SWELL1 or LRRC8a (leucine-rich repeat-containing protein 8a) encodes a transmembrane protein first described in 2003 as the site of a balanced translocation in an immunodeficient child with agammaglobulinemia and absent B-cells. So, for about a decade, SWELL1 was considered a membrane protein that regulates PI3K-AKT mediated lymphocyte function, and it was not until 2014 that SWELL1/LRRC8a was discovered to also form an essential component of the volume-regulated anion channel (VRAC), forming hetero-hexamers with LRRC8b-e22,23. We previously showed SWELL1 to mediate insulin-PI3K-AKT signaling in adipocytes, skeletal muscle, and endothelium via non-conductive signaling mechanisms. Also, we and others showed SWELL1-LRRC8 channel activity (conductive signaling) in the pancreatic β-cell is required for normal insulin secretion.

Additional binding interactions for SN-403, SN-406 and SN-407 are also predicted along the channel, due to the longer carbon chains affording additional hydrophobic interactions with side-chain carbons of the R103 residues (purple dashes). As anticipated, SN-403, SN-406, and SN-407 had increased ICl,SWELL inhibitory activity compared to SN-401, with SN-406 and SN-407 having IC50 of 3.1 and 1.6 μM, respectively, and SN-401 IC50 = 3.9 μM. In initial maps using sixfold symmetry, SN-407 density was less apparent than for DCPIB/SN-40131, potentially due to a reduction in SN-407 occupancy that is a consequence of lower compound solubility or the presence of multiple drug poses in different particles. In Pose-2, SN-407 is tilted off the SWELL1 central axis, positioning its cyclopentyl group closer to the hydrophobic cleft between SWELL1 subunits. These data confirm lengthening the carboxylate chain in SN-407 preserves electrostatic interactions with R103 and enables additional contacts between the carboxylate chain and upper hydrophobic moieties in distinct binding poses, consistent with the results of our docking simulations. However, collectively, these molecular docking, cryo-EM, and functional experiments indicate that SN-401 and SWELL1-active congeners (SN-403/406/407) bind to SWELL1-LRRC8 hexamers at both R103 (via carboxylate end) and at the interface between adjacent LRRC8 monomers (via hydrophobic end), to potentially stabilize the closed state of the channel, and thereby inhibit ICl,SWELL activity. Indeed, SN-401/SN-407 cryo-EM data and molecular docking simulations likely reflect the closed state of the SWELL1 homomer. Moreover, we hypothesize these SN-40X compounds may function as molecular tethers to stabilize assembly of the SWELL1-LRRC8 hexamer by binding between R103 and adjacent LRRC8 monomers, potentially reducing SWELL1-LRRC8 complex disassembly, subsequent proteasomal degradation, and thereby augment translocation from ER to plasma membrane signaling domains, akin to pharmacological chaperones.

>MIPVTELRYFADTQPAYRILKPWWDVFTDYISIVMLMIAVFGGTLQVTQDKMICLPCKWVTKDSCNDSFRGWAASSPEPTYPNSTVLPTPDTGPTGIKYDLDRHQYNYVDAVCYENRLHWFAKYFPYLVLLHTLIFLACSNFWFKFPRTSSKLEHFVSILLKCFDSPWTTRALSETVVEESDPKPAFSKMNGSMDKKSSTVSEDVEATVPMLQRTKSRIEQGIVDRSETGVLDKKEGEQAKALFEKVKKFRTHVEEGDIVYRLYMRQTIIKVIKFALIICYTVYYVHNIKFDVDCTVDIESLTGYRTYRCAHPLATLFKILASFYISLVIFYGLICMYTLWWMLRRSLKKYSFESIREESSYSDIPDVKNDFAFMLHLIDQYDPLYSKRFAVFLSEVSENKLRQLNLNNEWTLDKLRQRLTKNAQDKLELHLFMLSGIPDTVFDLVELEVLKLELIPDVTIPPSIAQLTGLKELWLYHTAAKIEAPALAFLRENLRALHIKFTDIKEIPLWIYSLKTLEELHLTGNLSAENNRYIVIDGLRELKRLKVLRLKSNLSKLPQVVTDVGVHLQKLSINNEGTKLIVLNSLKKMVNLTELELIRCDLERIPHSIFSLHNLQEIDLKDNNLKTIEEIISFQHLHRLTCLKLWYNHIAYIPIQIGNLTNLERLYLNRNKIEKIPTQLFYCRKLRYLDLSHNNLTFLPADIGLLQNLQNLAVTANRIEALPPELFQCRKLRALHLGNNVLQSLPSRVGELTNLTQIELRGNRLECLPVELGECPLLKRSGLVVEEDLFSTLPPEVKERLWRADKEQASNSLEVLFQ[6x]> SNTILGDLNDDGVVNGRDIVMMRQYLAGK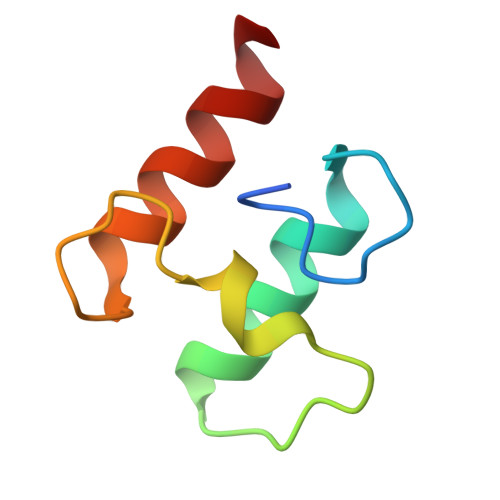TVSGIDKNALDINGDGAVNGDDLMELIKKVSNN[(1R)-4-phenyl-1-{[N-(pyrazine-2-carbonyl)-D-norvalyl]amino}butyl]boronic acid | C20 H27 B N4 O4 | 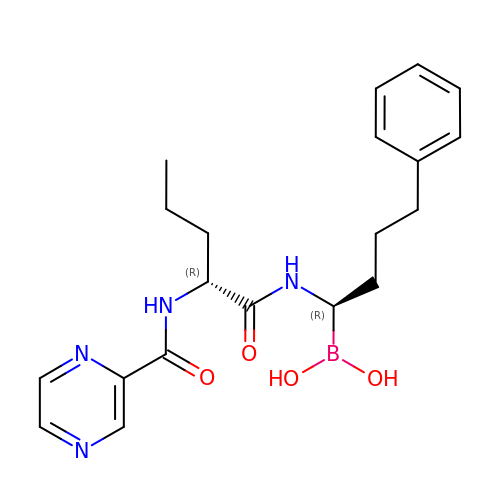KSQVGVMZECCPAT-AEFFLSMTSA-N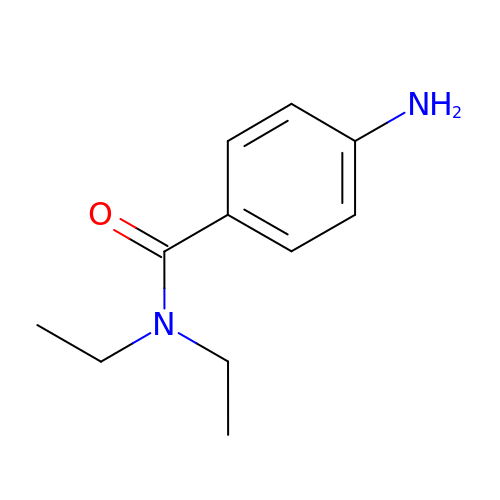4-amino-N,N-diethylbenzamide | C11 H16 N2 O | RNVOPVJRSRXPSX-UHFFFAOYSA-N3-methyl-5-{[5-(1-methylethyl)-2,6-dioxo-3-propyl-1,2,3,6-tetrahydropyrimidin-4-yl]carbonyl}benzonitrile 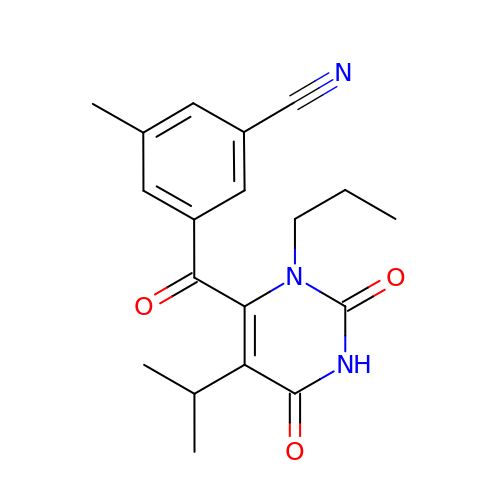| C19 H21 N3 O3 | ZXONPSZUOLSXSE-UHFFFAOYSA-N>MATIYFSSPLMPHNKKVQAVAGKRSTLLGVAQENGVKIPFECQDGNCGSCLVKITHLDGERIKGMLLTDKERNVLKSVGKLPKS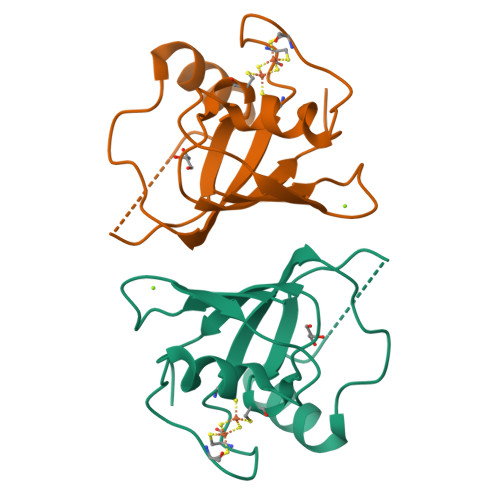EEERAAVRDLPPTYRLACQTIVTDEDLLVEFTGEPGGA[5x]>MGSINLRIDDELKARSYAALEKMGVTPSEALRLMLEYIADNERLPFKQTLLSDEDAELVEIVKERLRNPKPVRVTLDEL[3x];>MAYFLDFDERALKEWRKLGSTVREQLKKKLVEVLESPRIEANKLRGMPDCYKIKLRSSGYRLVYQVIDEKVVVFVISVGKAERSEVYSEAVKRIL[3x]

The bacterial relBE locus encodes a toxin-antitoxin complex in which the toxin, RelE, is capable of cleaving mRNA in the ribosomal A site cotranslationally. The antitoxin, RelB, both binds and inhibits RelE, and regulates transcription through operator binding and conditional cooperativity controlled by RelE. Binding of RelB inhibits RelE by displacement of the C-terminal, flexible α-helix, which contains a tyrosine residue (Tyr87) that is critical for catalysis (Li et al., 2009). RelB is additionally known to dimerize through formation of a ribbon-helix-helix (RHH) DNA binding motif that allows transcriptional autoregulation through binding to the relO operator region (Li et al., 2008; Overgaard et al., 2009).

In this work, we describe the crystal structure of the intact E. coli RelB2E2 TA complex determined to 2.8 Å resolution, corresponding to the fully RelE-saturated complex. The final structure comprises three RelBE heterodimers in the crystallographic asymmetric unit (ASU). Two of these heterodimers associate into a heterotetramer by noncrystallographic symmetry, and one engages in a similar interaction through a crystallographic 2-fold axis. The structure covers most of RelE (residues 2–80 of 95) and one molecule of RelB (residues 2–79 of 79), whereas the other two RelB molecules lack either the C terminus (residues 2–69) or N terminus (residues 33–79) due to poor electron density. The flexible, C-terminal helix of RelE (helix α3, residues 85–95) is disordered in all molecules in this crystal form. In the RelBE complex structure, each RelE tightly binds the C-terminal region of its associated RelB (residues 50–79) through displacement of helix α3 (Li et al., 2009). Two neighboring RelB molecules dimerize at their N termini to form a RHH-type DNA binding motif that closely resembles the structure of the isolated dimerization domain determined by nuclear magnetic resonance (NMR) (Li et al., 2008). In the resulting heterotetrameric complex, the extended conformation of helix α3 of RelB results in an overall very open, V-shaped complex with an RelE-RelB2-RelE architecture and approximate dimensions of 105 × 60 Å (top). At the position of Tyr87, which is required for the endonuclease activity of RelE, RelB has a valine (Val59∗), thus providing the hydrophobicity while removing the functional group. To understand the proposed model in structural terms, we used the structure of DNA-bound Arc to analyze the consequences of binding of the complete RelB2E2 tetramer to DNA. Structural alignment of two complete RelB2E2 tetramers with their RelB dimerization domains in adjacent major grooves immediately suggests why the complex cannot bind at high RelE concentrations: Due to the close proximity of the binding sites on DNA, binding of two adjacent tetramers generates an overlapping, W-shaped complex in which the two RelE molecules at each end of the complex (denoted as RelE and RelE′ in Figure S2A) clash.> AGTPDPLITEIQPWASEFGEAVDAHPYGLPIHFESHVKRQYVEWLTESPVSSINFTPIHALEGTITPQGCAFERHHSGAIELSKQDYRLMINGLVEKPLVFTFEDLLRFPRTTTTAFCECAANG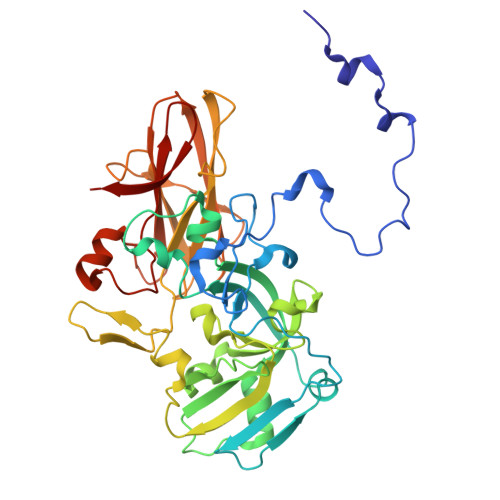GMEWGGAQLEGCQYTQGMIHNMEYVGVPLSVLLAEAGVKPEGKWLYAEGADASSNGRSFPMEKVMDDVMLAFFANGEALRKEHGYPARLVVPGWEGNMWVKWVRRLGIYDKAVESREETSKYTDLMPDGRARKWTWVMDAKSVITSPSPQVPIRHGKGPLVISGLAWSGNGRITRVDVSLDGGKNWTTARITGQALPKALTRFHLDIDWDGSEMLLQSRAVDETGYVQPTKDALRAIRGRNNVYHNNGIQTWWVKADGEVENVEIA>[2x]MFQMSETERTLVIIKPDAVVRGLIGEIISRFEKKGLKIVGMKMIWIDRELAEKHYEEHREKPFFKALIDYITKTPVVVMVLEGRYAVEVVRKMAGATDPKD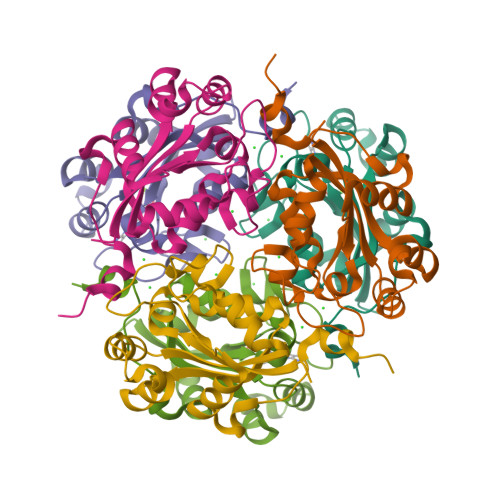AAPGTIRGDFGLEVSDAICNVIHASDSKESAEREISLFFKPEELFEYPRAADWFYKKGI>[2x]EDLDALWERYREAVRAGGNPQALYQEMVWPALLALWREKPRVYPFPQAFAVSVHTLGTSPEATALAILGAGAERVYVLHTPESARFLPRLRQDTGKDLYPVEIGKSDVEAIYREVKRLLEKHPEVPVALDLTSGTKAMSAGLAAAGFFFQRFYPKVRVVAVDNEDYDPELRRPRAGTEKLRILPNPHEALAEVDALFAKELYGKGEFGQAAAYFRGMVGRT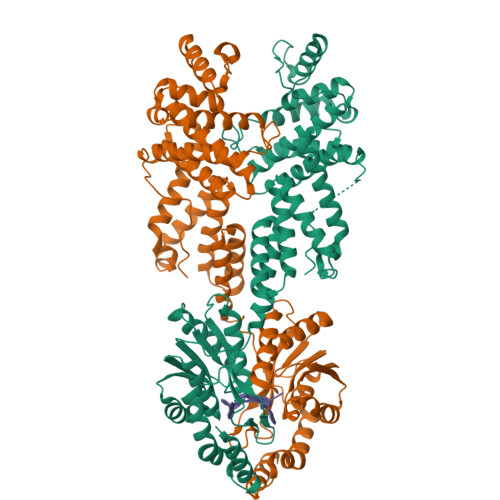GNQAYALYALLAEMYRAWRALDFGEALKAGRKLLGQLSQNVWLNHPLNARREALEAQVALLEAVDRFLKARDFALKEGVYGLARTLLHLAQEAKEEAAVLAALYAYRALELLLQERLALLGRRAEAPGLSPEEAEALRKALAELLGVLPEEVRLPAKLGLLDLLAFLRLKGDEALGRLSLAELRGLAGALKGRNSALLVHGFDVPSPKAVEGIARLAQGLLQDLEARTALGPLSPEPVPLGF> IVMPDGVTGKVPSLGWNSWNAYHCDIDESKFLSAAELIVSSGLLDAGYNYVNIDDCWSMKDGRVDGHIAPNATRFPDGIDGLAKKVHALGLKLGIYSTAGTATCAGYPASLGYEDVDAADFADWGVDYLKYDNCNVPSDW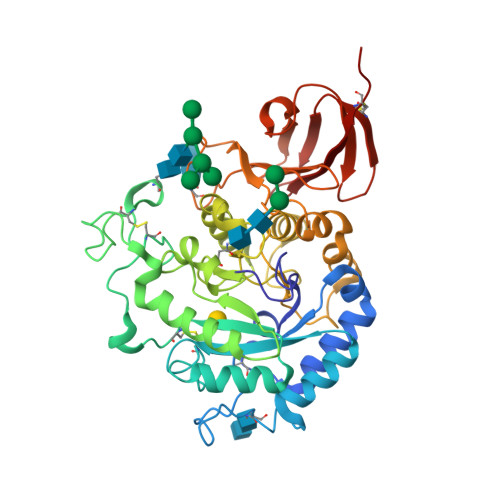QDEYVACNPDFVKTGPNGTCTTALDPTLAPPGYDWSTSKSAERFGAMRNALAKQSHEIVLSMCIWGQADVFSWGNSTGISWRMSDDISPNWGSVTRILNLNSFKLNSVDFWGHNDADMLEVGNGNLTAAETRTHFALWAAMKSPLLIGTDLAQLSQNNINLLKNKHLLAFNQDSVYGQPATPYKWGINPDWTFNVTYPAEFWAGPSSKGHLVLMVNTLDITATKEAKWNEIPGLSAGHYEVRDVWSDKDLGCLSSYKAAVAAHDTAVILVGKKCQRW>MRGSHHHHHHGSMDKNIIIGAMTALITPFKNGKVDEQSYARLIKRQIENGIDAVVPVGTTGESATLTHEENRTCIEIAVETCKGTKVKVLAGAGSNATHEAVGLAKFAKEHGADGILSVAPYYNKPTQQGLYEHYKAIAQSVDIPVLLYNVPGRTGCEISTDTIIKLFRDCENIYGV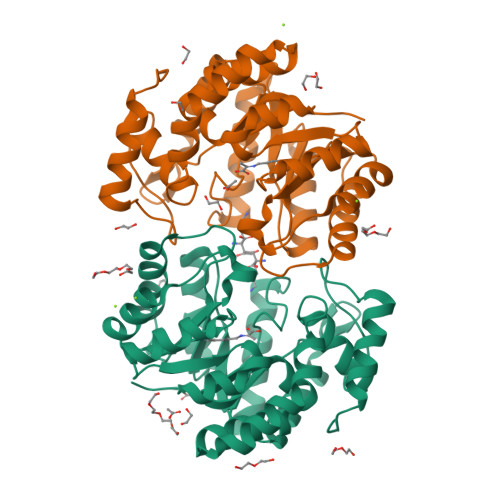KEASGNIDKCVDLLAHEPRMMLISGEDAINYPILSNGGKGVISVTSNLLPDMISALTHFALDENYKEAKKINDELYNINKILFCESNPIPIKTAMYLAGLIESLEFRLPLCSPSKENFAKIEEVMKKYKIKGF[6x]The RNase III enzyme Dicer-2 associates with its partner protein R2D2 and cleaves long double-stranded RNAs to produce 21-nucleotide siRNA duplexes, which are then loaded into Ago2 in a defined orientation. The Dicer-2–R2D2 heterodimer has critical roles in both siRNA production and siRNA loading onto Ago2. The present structures illuminated the detailed architectures of the individual domains and interdomain linkers of Dicer-2, which were not visible in the previous cryo-EM reconstructions at approximately 7 Å resolution, and revealed that Dicer-2 comprises an amino-terminal helicase domain, a DUF283 domain, a platform–PAZ domain, two RNase III domains (RIIIa and RIIIb) and a carboxy-terminal dsRNA-binding domain (CRBD). R2D2 comprises two dsRNA-binding domains (RBD1 and RBD2) and a carboxy-terminal domain (CTD).

We determined the cryo-EM structures of the Dicer-2–R2D2 heterodimer and the Dicer-2–R2D2–siRNA complex at 3.3 Å resolution. A structural comparison of Dicer-2–R2D2 and Dicer-2–R2D2–siRNA revealed that, although their overall structures are similar, the central linker becomes ordered and interacts with Dicer-2 CRBD and R2D2 RBD2 upon siRNA binding. R2D2 RBD1 in the Dicer-2–R2D2 structure was not resolved in the density map, suggesting that RBD1 is highly mobile in the siRNA-unbound state. R2D2 interacts with the helicase domain and the central linker of Dicer-2 to inhibit the promiscuous processing of microRNA precursors by Dicer-2. In particular, R324 and E331 of Dicer-2 form salt bridges with D288 and R223 of R2D2, respectively. A structural comparison of Dicer-2–R2D2 with DCL3–dsRNA suggested that Dicer-2 recognizes the 5′-monophosphate of dsRNA substrates in the 5′-pocket and cleaves the dsRNAs 21 nt away from the 5′ end in the RIIIb active site, consistent with a previous proposal. The modelled dsRNA sterically clashes with the helicase and CRBD domains of Dicer-2, suggesting that these domains undergo structural rearrangements upon the binding of dsRNA substrates.

> GSMEDVEIKPRGYQLRLVDHLTKSNGIVYLPTGSGKTFVAILVLKRFSQDFDKPIESGGKRALFMCNTVELARQQAMAVRRCTNFKVGFYVGEQGVDDWTRGMWSDEIKKNQVLVGTAQVFLDMVTQTYVALSSLSVVIIDECHHGTGHHPFREFMRLFTIANQTKLPRVVGLTGVLIKGNEITNVATKLKELEITYRGNIITVSDTKELENVMLYATKPTEVMVSFPHQEQVLTVTRLISAEIEKFYVSLDLMNIGVQPIRRSKSLQCLRDPSKKSFVKQLFNDFLYQMKEYGIYAASIAIISLIVEFDIKRRQAETLSVKLMHRTALTLCEKIRHLLVQKLQDMTYDDDDDNVNTEEVIMNFSTPKVQRFLMSLKVSFADKDPKDICCLVFVERRYTCKCIYGLLLNYIQSTPELRNVLTPQFMVGRNNISPDFESVLERKWQKSAIQQFRDGNANLMICSSVLEEGIDVQACNHVFILDPVKTFNMYVQSKGRARTTEAKFVLFTADKEREKTIQQIYQYRKAHNDIAEYLKDRVLEKTEPELYEIKGHFQDDIDPFTNENGAVLLPNNALAILHRYCQTIPTDAFGFVIPWFHVLQEDERDRIFGVSAKGKHVISINMPVNCMLRDTIYSDPMDNVKTAKISAAFKACKVLYSLGELNERFVPKTLKERVASIADVHFEHWNKYGDSVTATVNKADKSKDRTYKTECPLEFYDALPRVGEICYAYEIFLEPQFESCEYTEHMYLNLQTPRNYAILLRNKLPRLAEMPLFSNQGKLHVRVANAPLEVIIQNSEQLELLHQFHGMVFRDILKIWHPFFVLDRRSKENSYLVVPLILGAGEQKCFDWELMTNFRRLPQSHGSNVQQREQQPAPRPEDFEGKIVTQWYANYDKPMLVTKVHRELTPLSYMEKNQQDKTYYEFTMSKYGNRIGDVVHKDKFMIEVRDLTEQLTFYVHNRGKFNAKSKAKMKVILIPELCFNFNFPGDLWLKLIFLPSILNRMYFLLHAEALRKRFNTYLNLHLLPFNGTDYMPRPLEIDYSLKRNVDPLGNVIPTEDIEEPKSLLEPMPTKSIEASVANLEITEFENPWQKYMEPVDLSRNLLSTYPVELDYYYHFSVGNVCEMNEMDFEDKEYWAKNQFHMPTGNIYGNRTPAKTNANVPALMPSKPTVRGKVKPLLILQKTVSKEHITPAEQGEFLAAITASSAADVFDMERLEILGDSFLKLSATLYLASKYSDWNEGTLTEVKSKLVSNRNLLFCLIDADIPKTLNTIQFTPRYTWLPPGISLPHNVLALWRENPEFAKIIGPHNLRDLALGDEESLVKGNCSDINYNRFVEGCRANGQSFYAGADFSSEVNFCVGLVTIPNKVIADTLEALLGVIVKNYGLQHAFKMLEYFKICRADIDKPLTQLLNLELGGKKMRANVNTTEIDGFLINHYYLEKNLGYTFKDRRYLLQALTHPSYPTNRITGSYQELEFIGDAILDFLISAYIFENNTKMNPGALTDLRSALVNNTTLACICVRHRLHFFILAENAKLSEIISKFVNFQESQGHRVTNYVRILLEEADVQPTPLDLDDELDMTELPHANKCISQEAEKGVPPKGEFNMSTNVDVPKALGDVLEALIAAVYLDCRDLQRTWEVIFNLFEPELQEFTRKVPINHIRQLVEHKHAKPVFSSPIVEGETVMVSCQFTCMEKTIKVYGFGSNKDQAKLSAAKHALQQLSKCDA;> GPFTMDNKSAVSALQEFCARTQINLPTYSFIPGEDGGYVCKVELLEIEALGNGRSKRDAKHLAASNILRKIQLLPGIHGLMKDSTVGDLDEELTNLNRDMVKELRDYCVRREMPLPCIEVVQQSGTPSAPEFVACCSVASIVRYGKSDKKKDARQRAAIEMLALISSNSDNLRPDQMQVASTSKLKVVDMEESMEELEALRRKKFTTYWELKEAGSVDHTGMRLCDRHNYFKNFYPTLKKEAIEAINSDEYESSKDKAMDVMSSLKITPKISEVESSSLVPLLSVELNCAFDVVLMAKETDIYDHIIDYFRTMLI> SRVLLALHDRAPQLKISDDRLTVVGEKGYSMVRASHGVRKGAWYFEITVDEMPPDTAARLGWSQPLGNLQAPLGYDKFSYSWRSKKGTKFHQ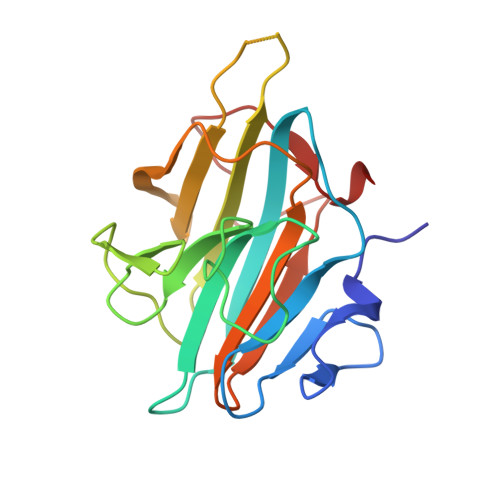SIGKHYSSGYGQGDVLGFYINLPEDTISGRGSSEIIFYKNGVNQGVAYKDIFEGVYFPAISLYKSCTVSINFGPCFKYPPKDLTYRPMSDMG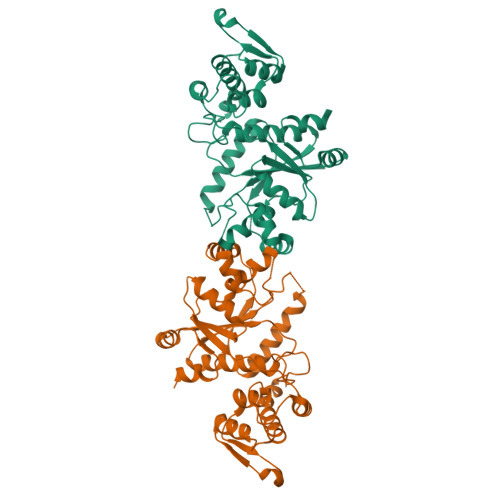>[2x]MDEFEMIKRNTSEIISEEELREVLKKDEKSASIGFEPSGKIHLGHYLQIKKMIDLQNAGFDIIIALADLHAYLNQKGELDEIRKIGDYNKKVFEAMGLKAKYVYGSEKHLDKDYTLNVYRLALKTTLKRARRSMELIAREDENPKVAEVIYPIMQVNGIHYKGVDVAVGGMEQRKIHMLARELLPKKVVCIHNPVLTGLDGEGKMSSSKGNFIAVDDSPEEIRAKIKKAYCPAGVVEGNPIMEIAKYFLEYPLTIKRPEKFGGDLTVNSYEELESLFKNKELHPMDLKNAVAEELIKILEPIRKRLLEHHHHHH>[2x]SNAMPLVSMKEMLNKALEGKYAVGQFNMNNLEWTQAILAAAEEEKSPVILGVSEGAARHMTGFKTVVAMVKALIEEMNITVPVAIHLDHGSSFEKCKEAIDA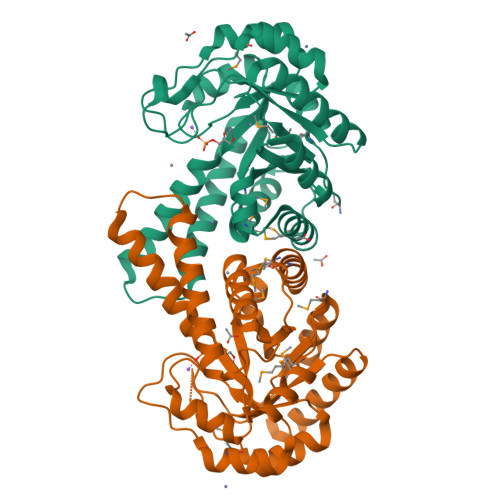GFTSVMIDASHHPFEENVETTKKVVEYAHARNVSVEAELGTVGGQEDDVIAEGVIYADPAECKHLVEATGIDCLAPALGSVHGPYKGEPNLGFAEMEQVRDFTGVPLVLHGGTGIPTADIEKAISLGTSKINVNTENQIEFTKAVREVLNKDQEVYDPRKFIGPGRDAIKATVIGKIREFGSNGKA4-ethyl-~{N}-[[1-[[(2~{R})-1-(1~{H}-indol-3-yl)-4-[[2-(methylamino)-2-oxidanylidene-ethyl]amino]-4-oxidanylidene-butan-2-yl]carbamoyl]cyclopropyl]methyl]benzamide | C29 H35 N5 O4 | 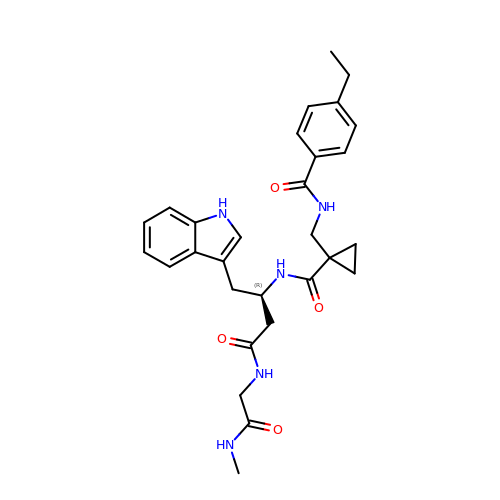HVVBCHJCCVHPJR-JOCHJYFZSA-N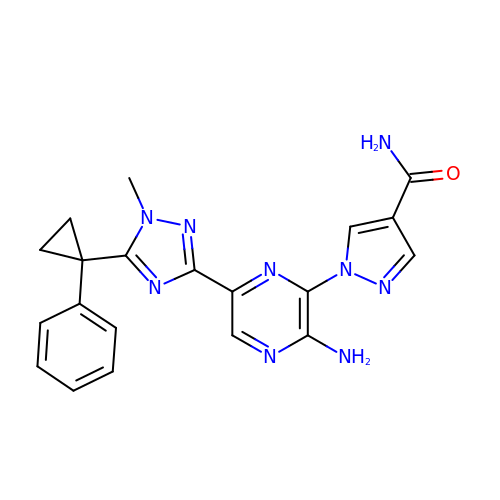1-[3-azanyl-6-[1-methyl-5-(1-phenylcyclopropyl)-1,2,4-triazol-3-yl]pyrazin-2-yl]pyrazole-4-carboxamide | C20 H19 N9 O | IYQNBZMEHITBAA-UHFFFAOYSA-N> APRSVALFHGIHPLNPKNYKTFSKEFETILNNAIEDGDFKGQLTEPCSYALRGGKYIRPIILMEIVRACQLQHSFGAPIYPAEAALAVEYFHVASLIIDDMPSFDNDVKRRNKDTVWARFGVAKAQMSALALTMQGFQNICRQIDWIKEHCPRFPDPNQLGALLCTFVSHSLNSAGSGQLVDTP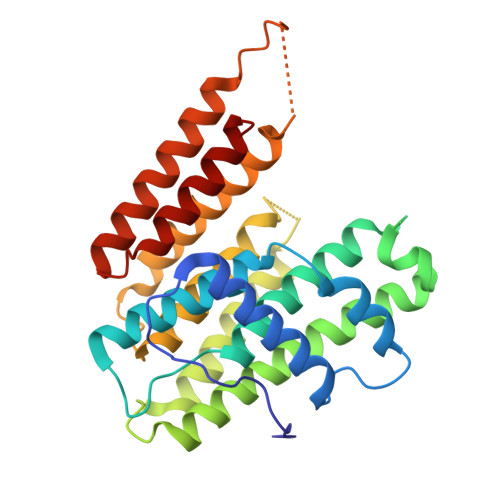EKTIPFFKIAFIMGWVLGTGTIEDIGMIERAAHCFGHAFQLADDIKDHDTDTGWNYAKIHGKQKTFDDVAQSLQECKKILHGKKIFTSIWNEIFQKVINVALGT methyl (2E,6E)-9-[(2R,3S)-3-ethyl-3-methyloxiran-2-yl]-3,7-dimethylnona-2,6-dienoate | C17 H28 O3 | 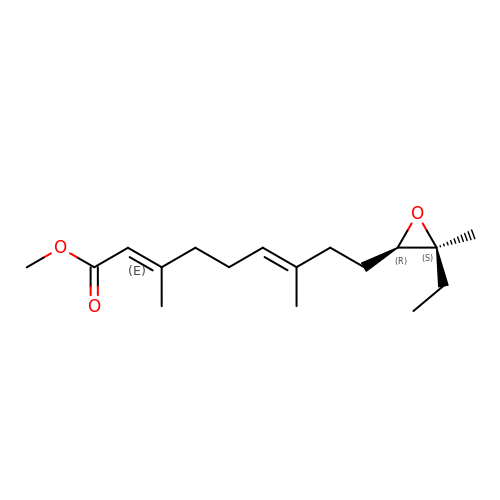CPVQJXZBSGXTGJ-TZDLBHCHSA-N> PISPIETVPVKLKPGMDGPKVKQWPLTEEKIKALVEICTEMEKEGKISKIGPENPYNTPVFAIKKKDSTKWRKLVDFRELNKRTQDFWEVQLGIPHPAGLKKKKSVTVLDVGDAYFSVPLDEDFRKYTAFTIPSINNETPGIRYQYNVLPQGWKGSPAIFQSSMTKILEPFKKQNPDIVIYQYMDDLYVGSDLEIGQHRTKIEELRQHLLRWGLTTPDKKHQKEPPFLWMGYELHPDKWTVQPIVLPEKDSWTVNDIQKLVGKLNWASQIYPGIKVRQLSKLLRGTKALTEVIPLTEEAELELAENREILKEPVHGVYYDPSKDLIAEIQKQGQGQWTYQIYQEPFKNLKTGKYARMRGAHTNDVKQLTEAVQKITTESIVIWGKTPKFKLPIQKETWETWWTEYWQATWIPEWEFVNTPPLVKLWYQLEKEPIVGAETFYVDGAANRETKLGKAGYVTNKGRQKVVPLTNTTNQKTELQAIYLALQDSGLEVNIVTDSQ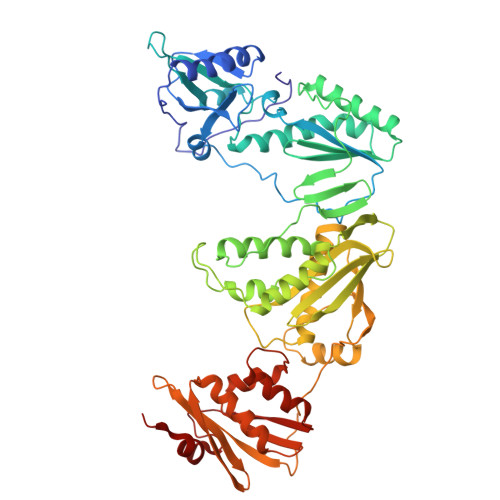YALGIIQAQPDKSESELVNQIIEQLIKKEKVYLAWVPAHKGIGGNEQVDKLVSAGI>[2x]SNAYLPKHESVTLKNGLQVVSVPLENKTGVIEVDVLYKVGSRNEVMGKSGIAHMLEHLNFKSTKNLKAGEFDKIVKRFGGVSNASTSFDITRYFIKTSEANLDKSLELFAETMGSLNLKEDEFLPERQVVAEE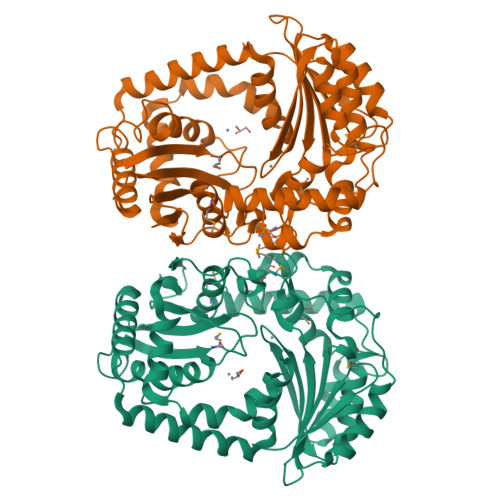RRWRTDNSPIGMLYFRFFNTAYVYHPYHWTPIGFMDDIQNWTLKDIKKFHSLYYQPKNAIVLVVGDVNSQKVFELTKKHFESLKNLDEKAIPTPYMKEPKQDGARTAVVHKDGVHLEWVALGYKVPAFKHKDQVALDALSKLLGEGKSSWLQSELVDKKRLASQAFSHNMQLQDESVFLFIAGGNPNIKAEALQKEIVALLEKLKKGEITQAELDKIKINQKADFISNLESSSDVAGLFADYLVQNDLQGLTDYQQQFLDLKVSDLVRVANEYFKDTQSTTVFLKP>[4x]FQSMNRSALDFRHFVDHLRRQGDLVDVHTEVDANLEIGAITRRVYERRAPAPLFHNIRDSL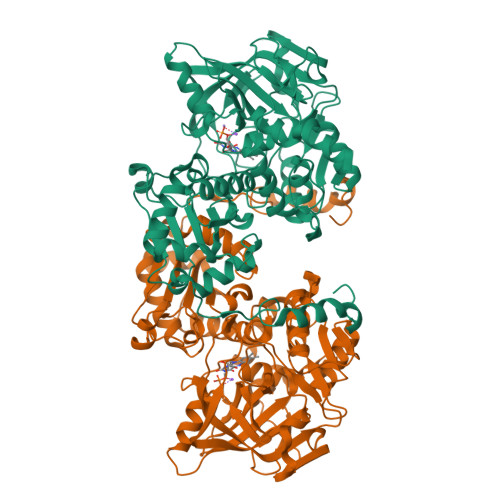PGARVLGAPAGLRADRARAHSRLALHFGLPEHSGPRDIVAMLRAAMRAEPIAPRRLERGPVQENVWLGEQVDLTRFPVPLLHEQDGGRYFGTYGFHVVQTPDGSWDSWSVGRLMLVDRNTLAGPTIPTQHIGIIREQWRRLGKPTPWAMALGAPPAALAAAGMPLPEGVSEAGYVGALVGEPVEVVRTQTNGLWVPANTEIVLEGEISLDETALEGPMGEYHGYSFPIGKPQPLFHVHALSFRDQPILPICVAGTPPEEHHTIWGTMISAQLLDVAQNAGLPVDMVWCSYEAATCWAVLSIDVQRLAALGTDAAAFAARVAETVFGSHAGHLVPKLILVGNDIDVTEIDQVVWALATRAHPLHDHFAFPQIRDFPMVPYLDAEDKARGSGGRLVINCLYPEQFAGQMRAATASFRHAYPTALRRRVEERWSDYGFGDA>MRGSHHHHHHGSMRMKYNVEEKGTKVIVRGIADFNLKETFESGQCFRWNEEEDGSYTGVAYDRVVNVKLEGDTLIIDNTNLTDFYDIWFDYFDLGRDYGQIKESLSKDPVLKEAIKFGQGIRILRQDTWETLVSFIVSQNNRIPQIKKVIENLATSFGNPIEYKGKIYYTFPKPEELVMYDVETIAKTRCGF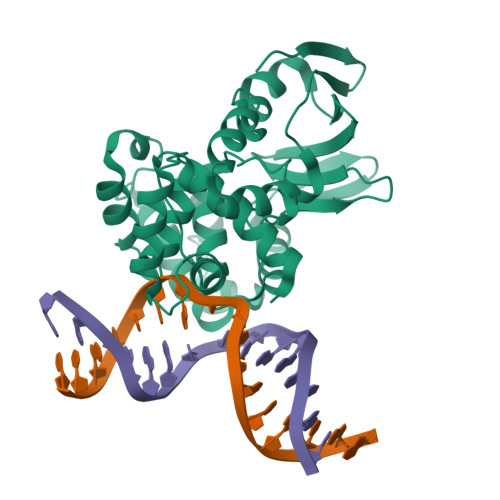RAKYIFDAASKVFSGEINLLKLHEYSTSEIRDILMTINGVGPKVADCVILYSIGRYDTFPTDVWIKRIVEHLYLKREGTPVEIQLFAIDKFGDLSGFAQQYLFYYGREMGKKIFGERKK[2x]>[2x]XELAQAFKEIAKAFKEIAKAF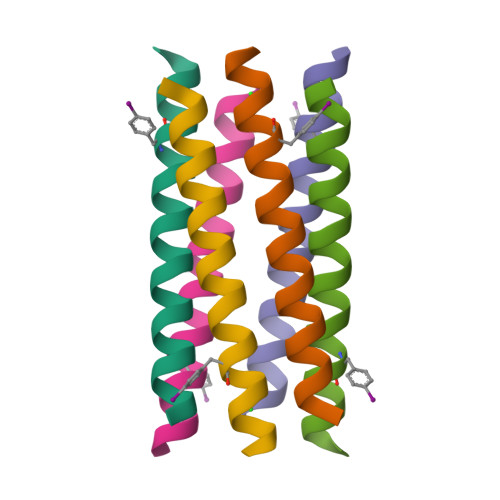EFIAQAIEKX>MIAELFTNNALNLVIIFGSCA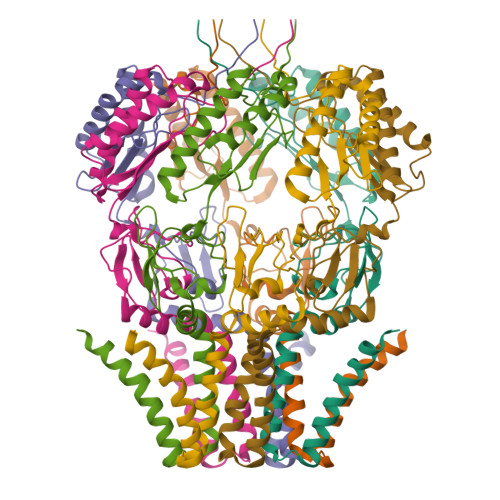ALILMSFWFRRGNRKRKGFLFHAVQFLIYTIIISAVGSIINYVIENYKLKFITPGVIDFICTSLIAVILTIKLFLLINQFEKQQIKKGRDITSARIMSRIIKITIIVVLVLLYGEHFGMSLSGLLTFGGIGGLAVGMAGKDILSNFFSGIMLYFDRPFSIGDWIRSPDRNIEGTVAEIGWRITKITTFDNRPLYVPNSLFSSISVENPGRMTNRRITTTIGLRYEDAAKVGVIVEAVREMLKNHPAIDQRQTLLVYFNQFADSSLNIMVYCFTKTTVWAEWLAAQQDVYLKIIDIVQSHGADFAFPSQTLYMDNITPPEQGRHHHHHH[7x]2,6-bis(bromanyl)phenol | C6 H4 Br2 O | 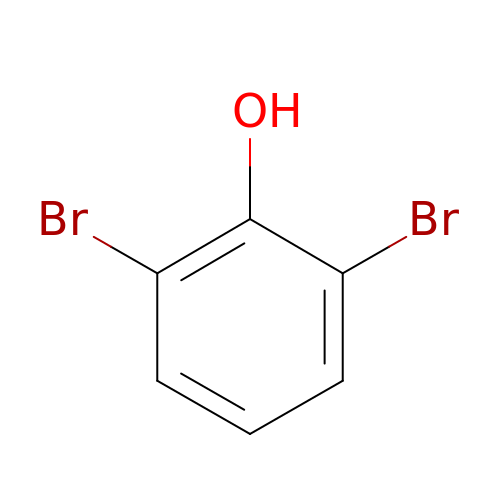SSIZLKDLDKIHEV-UHFFFAOYSA-N In the Gram-positive model bacterium Bacillus subtilis, TasA is the major protein component of the biofilm matrix, where it has been reported to form functional amyloid fibres contributing to biofilm structure and stability. Here, we present electron cryomicroscopy structures of TasA fibres, which show that, rather than forming amyloid fibrils, TasA monomers assemble into fibres through donor-strand exchange, with each subunit donating a β-strand to complete the fold of the next subunit along the fibre. Later studies revealed that TasA assembles into fibres that form the major component of the B. subtilis biofilm matrix, with deletions of tasA resulting in significant defects in biofilm and pellicle formation that can be rescued by addition of exogenous TasA17. The structure of TasA fibres reveals that the TasA system is a donor-strand exchange system in Gram-positive bacteria.

To gain insights into the structure of TasA fibres, we purified TasA from a B. subtilis double mutant strain (∆sinR ∆eps) that lacks the matrix polysaccharide operon eps, thereby producing TasA that is not associated with EPS, as well as the regulator gene sinR, an eps and tasA repressor, causing the strain to overproduce TasA17. We performed helical reconstruction from cryo-EM images and determined a 3.5 Å resolution structure of TasA fibres. Interestingly, this structure shows that TasA monomers polymerise into fibres through an N-terminal β-strand that extends from each subunit into the next. There, this extended ‘donor strand’ completes a β-sheet of the following (n + 1)th subunit, and in this way provides an extensive inter-subunit interaction. In addition to the β-sheet hydrogen bonding of the donor strand with the next subunit, there are extensive hydrophobic interactions between donor strand residues (F29, I32, F39) and the next two subunits. The C-terminal residues 239–261, previously found to be unstructured in NMR studies of monomeric TasA and not present in the monomer X-ray structure, are ordered in the fibre structure and form another inter-subunit interface. Remarkably, we observed that the binding site of the donor strand is self-complemented by a different β-strand (residues 48–61) in the monomeric form. In the fibre form, the previously self-complementing β-strand (residues 48–61) is displaced by the donor strand of the (n-1)th subunit (residues 28–38). The previously self-complementing strand then folds over the opposite β-sheet, and the donor strand (residues 28–38), along with residues 39–47, extends towards the next (n + 1)th subunit, allowing assembly of the next subunit. Thus, the fibre structure is neither representative of cross-β amyloids, nor is it a head-to-tail arrangement of globular subunits as previously suggested, but shares features of both, including inter-subunit interactions mediated by β-strands and an intact core fold of the monomer.

>AFNDIKSKDATFASGTLDLSAKENSASVNLSNLKPGDKLTKDFQFENNGSLAIKEVLMALNYGDFKANGGSNTSPEDFLSQFEVTLLTVGKEGGNGYPKNIILDDANLKDLYLMSAKNDAAAAEKIKKQIDPKFLNASGKVNVATIDGKTAPEYDGVPKTPTDFDQVQMEIQFKDDKTKDEKGLMVQNKYQGNSIKLQFSFEATQWNGLTIKKDHTDKDGYVKENEKAHSEDKN[3x]> TEFKAGSAKKGATLFKTRCLQCHTVEKGGPHKVGPNLHGIFGRHSGQAEGYSYTDANIKKNVLWDENNMSEFLTNPKKY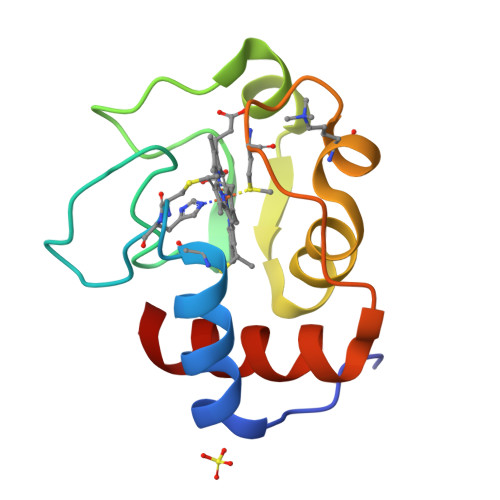IPGTKMAFGGLKKEKDRNDLITYLKKATE Immature retroviruses are built by the Gag polyprotein; Gag is then cut into domains, and the resulting CA capsid proteins form the mature capsid, which can mediate infection of a new cell. Murine leukemia virus (MLV), the prototypic member of the γ-retroviruses, is commonly used in comparative studies and as a basis for retroviral vector design. The CA domain and immediate downstream residues mediate protein interactions in the immature shell, and, following proteolytic cleavage, CA forms the mature viral capsid. In this study, we have determined the structure of the truncated MLV CA-CTD by X-ray crystallography and have resolved the architecture and CA lattice structures of immature and mature MLV particles by cryo-ET and subtomogram averaging.

Purified mature, infectious MLV particles from the culture medium of transfected HEK293T cells were inactivated and subjected to cryo-ET, and 134 mature viruses were identified in 65 tomograms. We applied subtomogram averaging to obtain a density map of the CA hexamer in the core of the mature virions at 7.2-Å resolution. As previously described for HIV-1, the mature MLV CA lattice is thinner than the immature Gag shell, consisting of a single layer including CA-NTD and CA-CTD. The hexamer–hexamer spacing in the middle of the mature CA layer was 10.0 ± 0.4 nm, consistent with previous measurements from HIV-1 (28), and larger than that in the immature virus. The CA-CTD interacts at the twofold axes via helix 9 (black arrow), as seen in other retroviruses, but also via interactions between K201 in helix 310b and D171 in the loop between helices 8 and 9 (black arrowhead). As for HIV-1, in mature MLV, there is a CA-CTD–CA-NTD interface. This involves helix 4 and helix 8 (asterisk). The observed density extends beyond the C terminus of the truncated protein used for crystallography in a short rod-shaped density toward the center of the core (red arrowhead). This density would accommodate an α-helix corresponding approximately to residues P222–R230 of the CAH. Three of these short helices cluster around the threefold symmetry axis, bringing their C-terminal ends toward one another (red arrowhead, triangle).

>[3x]PLRMGGNGQLQYWPFSSSDLYNWKNNNPSFSEDPGKLTALIESVLTTHQPTWDDCQQLLGTLLTGEEKQRVLLEARKAVRGNDGRPTQLPNEVDAAFPLERPDWDYTTQRGRNHLVLYRQLLLAGMQNAGRSPTNLAKVKGITQGPNESPSAFLERLKEAYRRYTPYDPEDPGQETNVSMSFIWQSAPDIGRKLERLEDLKSKTLGDLVREAEKIFNKRETPEEREERIRRETEEK> MLDRLDAALRFQQEALNLRAQRQEILAANIANADTPGYQARDIDFASELKKVMVRGREETGGVALTLTSSHHIPAQAVSSPAVDLLYRVPDQPSLD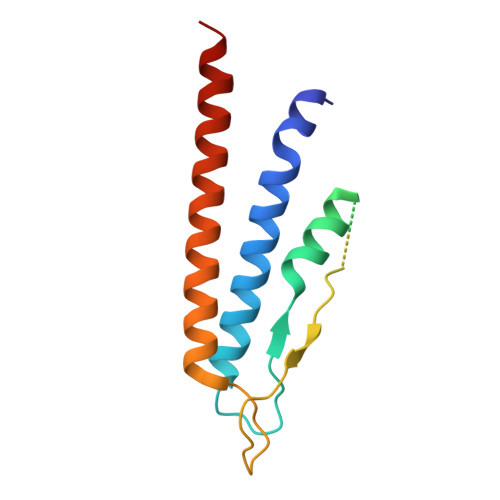GNTVDMDRERTQFADNSLKYQMGLTVLGSQLKGMMNVLQGGN>SATSAHSFTGRPLHIPPLPCPFPSEINEHADAVDEESHTWLAASHMLKGADTVEHFRRSKIGTLAARTNPTVPRDSLRLIND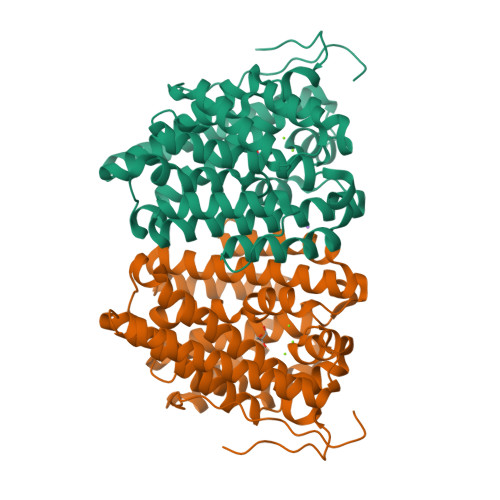WYNWLFAFDDAFCEGELMGHRASALARALPPLLEILDGRREPDGSDAFGLALKELLHRISDVASPAQVDRWRTTVKEYLFAQIWEAANREVDLIPTPDDYVLMRRITGATYTCFALIDVGGGYRLEAEEWHHPDVRTLSDLACDLIGWDNDLLSYAKERGNDKARHNLVTVLATHKSLTLQDALLEVAQMHNDAVAAFLDRRAALDRWATLPVRKYVRGLEHWVRGHIAFSLGSARYVGAWPDDTRWPRAV[2x]> SNAVKRKGVEVMIALDISNSMLAQDVQPSRLEKAKRLISKLVDGMENDKVGMIVFAGDAFTQLPITSDYISAKMFLESISPSLISKQGTAIGAAINLAARSFTPQEGVGRAIVVITDGENHEGGAVAAAKSSSSSGIQVNVLGVGLPDGAPIPIEGSNDFRRDREGNVIVTRLNEAMCQEIAKEGNGIY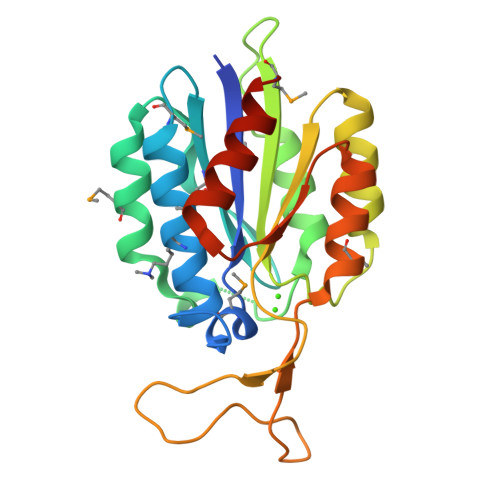IRVDNSNSAQKAINQEINKMAKSDVE In the present study, we identified and isolated choline-binding protein A (CbpA) as an S-layer protein of L. salivarius REN that we show is important for adhesion. The adhesion values of ΔcbpA and Δnam-amidase mutants to HT-29 cells were reduced by 62% and 16%, respectively, compared with wild-type (WT), indicating that CbpA represents the major surface adherence factor of L. salivarius REN. CbpA may represent a new class of surface layer proteins, which contain an N-terminal domain required for cell wall-anchoring through choline binding and an M23 family peptidase C-terminal domain required for the interaction with the ENO1 receptor on the surface of host cells. Here, the results of our in vitro binding and co-immunoprecipitation experiments show that enolase is the CbpA receptor expressed by HT-29 cells.

The structure of CbpA was solved at 1.85 Å resolution. The structure comprises residues 360–512, and residues 338–359 were not visible in the electron density map. The entire structure, which shares key features with those of M23-family peptidases, includes a central six-stranded antiparallel β-sheet (β1, β3, β4, β5, β6 and β8) that forms a “sandwich” structure, two other β-sheets (β2 and β7) are packed against the bottom of the β-sheet and helices α1 and α2 in the C-terminus pack against the top. The core antiparallel β-sheet anchors the catalytic residues, which bind a central Zn2+. Zn2+ is coordinated by three adjacent residues (His395, Asp399 of the characteristic HxxxD motif and His475 of the HxH motif) and three water molecules (W110, W111 and W119) in a nearly perfect octa-hedral arrangement. Glu444 and His473 interact with the metal ion through the W111 water molecule. CbpA contains a longer L-shaped Loop 1 above the Zn2+, thus forming a lid above the active site that regulates the entrance of the substrate towards the middle of the groove. It differs most in the loop 4 of CbpA, forming an α-helix rather than a coil that is present in lysostaphin. These different conformations of the loops in CbpA may indicate binding to more diverse substrates compared with lysostaphin. In the active site of CbpA, the corresponding anionic center that coordinates the lysine residues of ENO1 may include Asp396 and Asp399, and the binding of the cationic to the carboxylate moiety of ENO1 may require Arg390.

> MGSSHHHHHSSGENLYFQGGSKDTWGWPFPSVGEGYFSGAQLFGVNPGGEFRMNGFHDGLDFGSIDHPGSAVHAVHSGVVTQIGYIAGLENYVVVRSDEYTFVYQEAFSNKGNISVKVGQQINTGDVIGYRDTSHLHLGITRETNVMKAIANSFNNNGTWLDPRALIKNGIANQ> GSARGMALYEEEQVERIGDIEERGKILVSLMYSTQQGGLIVGIIRCVHLAAMDANGYSDPFVKLWLKPDMGKKAKHKTQIKKKTLNPEFNEEFFYDIKHSDLAKKSLDISV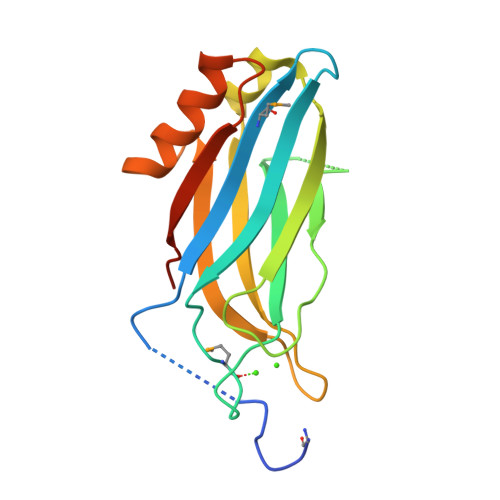WDYDIGKSNDYIGGCQLGISAKGERLKHWYECLKNKDKKIERWHQLQNENHVSSD>[4x]MLGTSGVKIHPNGNSNQLGVQLENVKLTSLFKKLDKRCSLASWIKENIKKKECCFYVEDGREGICKCGYPKVQHCDEAIKPEDYMGEQWDKHRHVRETPTDAFGDISFGGLGQKTGKYVRVSSDTSCENLYQLMTEQWKLRSPNLLISVTGGAKNFYIKTHLKDKFRRGLIKVAQTTGAWILTGGTHAGVMKHVGMAVRDYTLSSGSMEGQIVVIGVAPWGVIHNRSTLIHPEGRFPAYYSLDEQGQGRLSCLDINHTHFLLVDDGTQGHYGVEIELRARLEKLISKLSLGNRESGVTIPVVCVVLDGGPGTLNTIYNSMLNHTPCVVLEGSGRLADVIAHVASVPVSKVTMALINRLLKRFFMQEYKNFTELQIIEWTKKIQDILRMPHLLTVFRIDEDKNYDVDVAILQALLKASRSDEHAGRHCWERQLELAVAWNRVDIAESEIFTEESQWTSSDLHPAMFSALVGDKPEFVRLLLENGVCVREFLEREETLCELYSHLPSCFFLRKLAKRVQGGKMRRGQEPLPGSRKVCLSHVSEEVRHLLGSFTQPLYIASRYKPTKDDVRLKVPSKGALDLPCSGEEWSADTVWDPGRDLFLWAVVQNNRELAEIGWEQCRDCIAAALAASKILRKLAQESGEDDSEEATEMLELANHYEKQAIGVFSECHSWDAQRAQKLLIRISPSWGRSTCLWLALEAHDKSFIAHSGVQALLTQIWCGELSVDNPHWKVLLCMIFFPLIYTGFLTFRRDEDIQRQAERTQQKLAMESVFAGQSDGKIKRHLRGFSQKSELKPLNCSSRLMSFLKSPQVKFYWNIASYFGFLWLFAVVLMIDFQTSPSWRELLLYVWLTSLVCEEIRQLYHDFDGSGFRRKAKMYIKDLW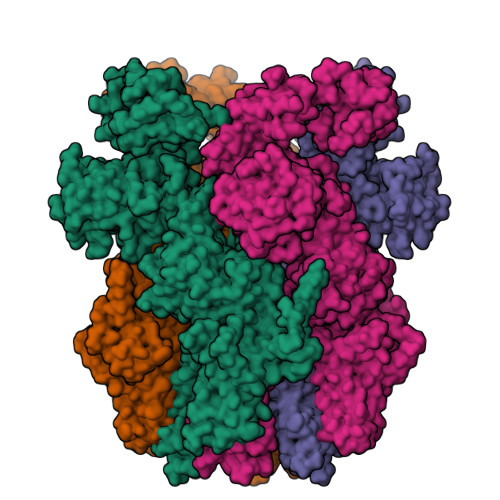NILDVLSIVLFIAGLICRLQASDTVFYIGKVILCIDFIIFCLRLMAIFSISRTLGPKIIIVRRMMLDLFFFMFLLSIWVVAYGVAKQGILIENEERLNWIIRGAVYEPYITIFGNFPTNIDNTLFDISSCSVNASDPLKPKCPMLNADNTPVFPEWLTIMMLCVYLLFANILLLNLLIAIFNYTFQEVQDNTDTIWKFQRYELIKEYHSRPALPPPFILLSHLILFIRGVFLRDLPQRHKNFRQELEQTEEEELLSWEAYMKDNYLASTRQDESQSVEHRIHDTAEKVGAMSELLEREQEMVSATMAKRLARLEEQVSESAKALRWIIDALKSQGCKSKVQPPLMRSKSSDRDDGDSSGQETDDEEAPHMFARQLQYPDSTVRRFPVPEEKVSWEVNFSPYQPPVYNQQDSSESDTSALDKHRNPGGRTGIRGKGALNTLGPNHILHPIFTRWRDAEHKVLEFLAVWEDAEKRWALLGGPAQPDEPLAQVLERILGKKLNEKTKTLLKAGEEVYKGYVDDSRNTDNAWVETSIITLHCDKNTPLMADLNHMVESSLSSHQPLQWREVSSDACRCSYQREALRQIAHHHNTYF>PFTYSIEATRNLATTERCIQDIRNAPVRNRSTQFQLAQQNMLAYTFGEVIPGFASAGINGMDYRDVIGRPVENAVTEGTHFFRDDFRVDSNAKAKVAGDIFEIVSSAVMWNCAARWNSLMVGEGWRSQPRYSRPTLSPSPRRQVAVLNLPRSFDWVSLLVPESQEVIEEFRAGLRKDGLGLPTSTPDLAVVVLPEEFQNDEMWREEIAGLTRPNQILLSGAYQRLQGRVQPGEISLAVAFKRSLRSDRLYQPLYEANVMQLLLEGKLGAPKVEF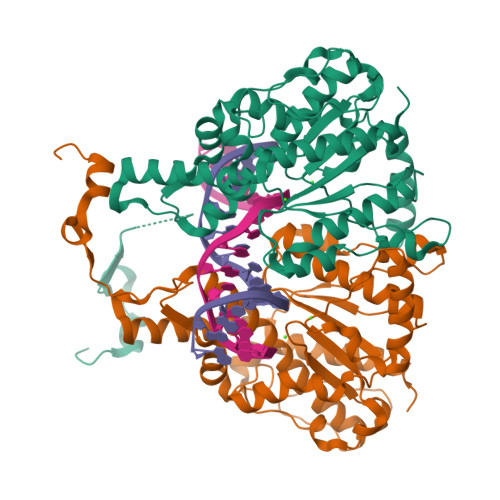EVHTLAPEGTNAFVTYEAASLYGLAEGRSAVHRAIRELYVPPTAADLARRFFAFLNERMELVNG[8x]[(2S,3R,4R)-4-(6-amino-9H-purin-9-yl)oxetane-2,3-diyl]dimethanol 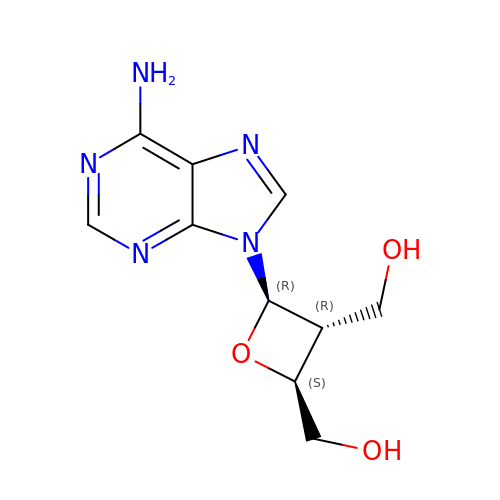| C10 H13 N5 O3 | LMJVXGOFWKVXAW-OXOINMOOSA-N> GPLGSPEFMTWPVKDFNYSDPVNDNDILYLRIPQNKLITTPVKAFMITQNIWVIPERFSSDTNPSLSKPPRPTSKYQSYYDPSYLSTDEQKDTFLKGIIKLFKRINERDIGKKLINYLVVGSPFMGDSSTPEDTFDFTRHTTNIAVEKFENGSWKVTNIITPSVLIFGPLPNILDYTASLTLQGQQSNPSFEGFGTLSILKVAPEFLLTFSDVTSNQSSAVLGKSIFCMDPVIALMHELTHSLHQLYGINIPSDKRIRPQVSEGFFSQDGPNVQFEELYTFGGLDVEIIPQIERSQL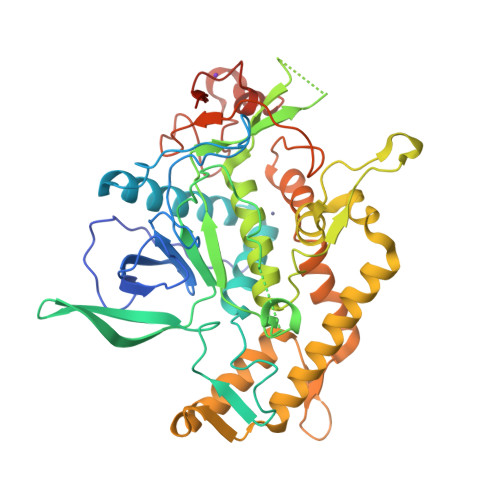REKALGHYKDIAKRLNNINKTIPSSWISNIDKYKKIFSEKYNFDKDNTGNFVVNIDKFNSLYSDLTNVMSEVVYSSQYNVKNRTHYFSRHYLPVFANILDDNIYTIRDGFNLTNKGFNIENSGQNIERNPALQKLSSESVVDLFTKV>[2x]MSNSYEGCGDLTIFVAVALNKVIGHKNQIPWPHITHDFRFLRNGTTYIPPEVLSKNPDIQNVVIFGRKTYESIPKASLPLKNRINVILSRTVKEVPGCLVYEDLSTAIRDLRANVPHNKIFILGGSFLYKEVLDNGLCDKIYLTRLNKEYPGDTYFPDIPDTFEITAISPTFSTDFVSYDFVIYERKDCKTVFPDPPFDQLLMTGTDISVPKPKYVACPGVRIRNHEEFQYLDILADVLSHGVLKPNRTGTDAYSKFGYQMRFDLSRSFPLLTTKKVALRSIIEELLWFIKGSTNGNDLLAKNVRIWELNGRRDFLDKNGFTD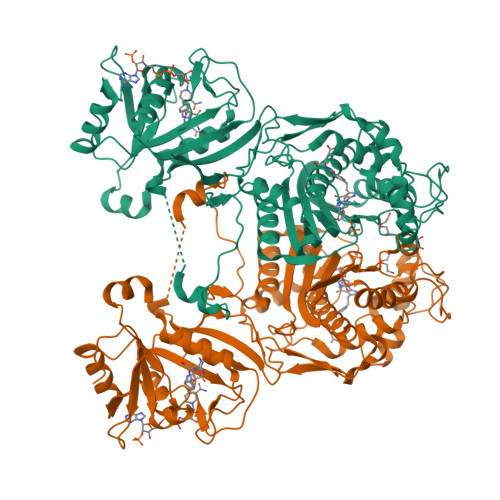REEHDLGPIYGFQWRHFGAEYLDMHADYTGKGIDQLAEIINRIKTNPNDRRLIVCSWNVSDLKKMALPPCHCFFQFYVSDNKLSCMMHQRSCDLGLGVPFNIASYSILTAMVAQVCGLGLGEFVHNLADAHIYVDHVDAVTTQIARIPHPFPRLRLNPDIRNIEDFTIDDIVVEDYVSHPPIPMAMSA> ADCAKGKIEFSKYNENDTFTVKVAGKEYWTNRWNLQPLLQSAQLTGMTVT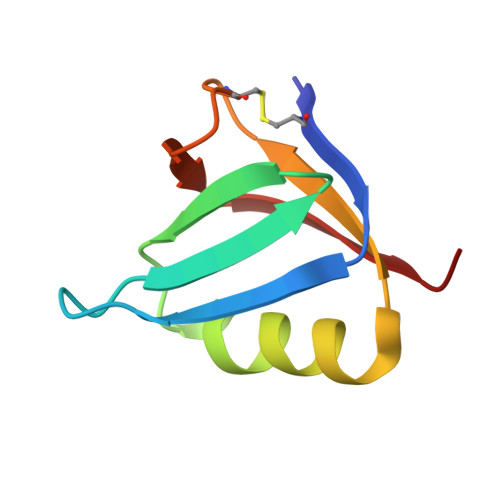IKSSTCASGSGFAEVQFNND1-(furan-2-ylmethyl)-5-(trifluoromethyl)benzimidazol-2-amine 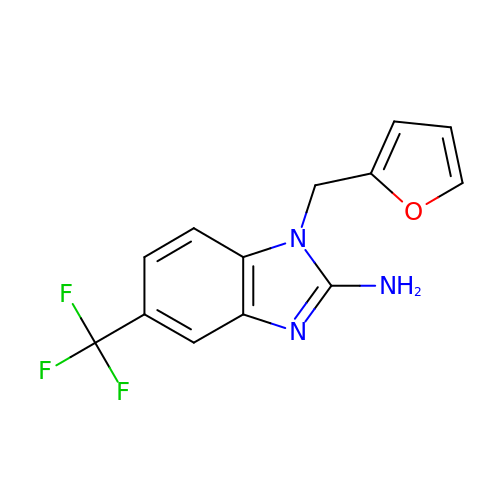| C13 H10 F3 N3 O | QYVPLFHAOLRMBY-UHFFFAOYSA-N> PPLHDFYCSRLLDLVFLLDGSSRLSEAEFEVLKAFVVDMMERLRISQKWVRVAVVEYHDGSHAYIGLKDRKRPSELRRIASQVKYAGSQVASTSEVLKYTLFQIFSKIDRPEASRITLLLMASQEPQRMSRNFVRYVQGLKKKKVIVIPVGIGPHANLKQIRLIEKQAPENKAFVLS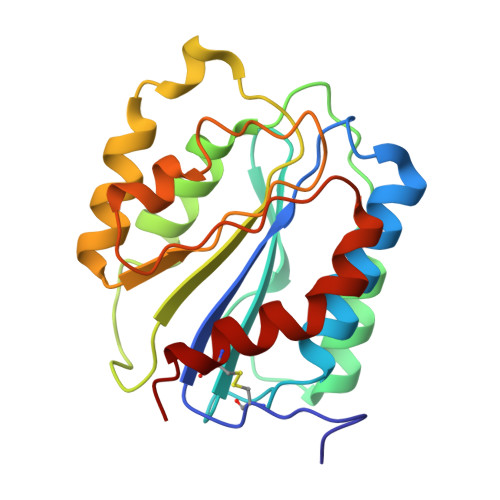SVDELEQQRDEIVSYLCDLAPE> DTAPT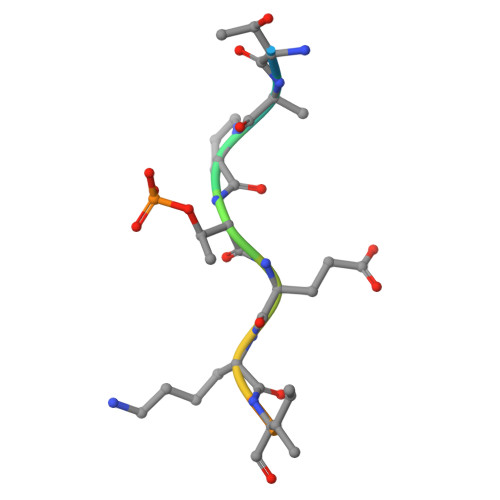EKIAYKK>[2x]AFGKLHPTNPEVTMNISQMITYWGYPAEEYEVVTEDGYILGIDRIPYGRKNSENIGRRPVAFLQHGLLASATNWISNLPNNSLAFILADAGYDVWLGNSRGNTWARRNLYYSPDSVEFWAFSFDEMAKYDLPATIDFILKKTGQDKLHYVGHSQGTTIGFIAFSTNPKLAKRIKTFYALAPVATVKYTETLINKLMLVPSFLFKLIFGNKIFYPHHFFDQFLATEVCSRETVDLLCSNALFI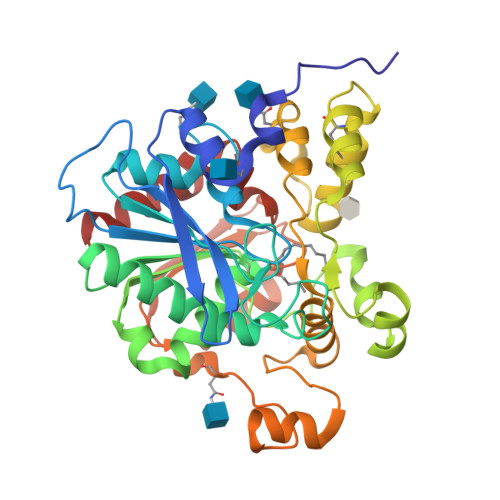ICGFDTMNLNMSRLDVYLSHNPAGTSVQNVLHWSQAVKSGKFQAFDWGSPVQNMMHYHQSMPPYYNLTDMHVPIAVWNGGNDLLADPHDVDLLLSKLPNLIYHRKIPPYNHLDFIWAMDAPQAVYNEIVSMMGTD>APDSVDYREKGYVTPVKNQGQCGSCWAFSSVGALEGQLKKKTGKLLNLSPQNLVDCVSENDGCGGGYMTNAFQYVQKNRGIDSEDAYPYVGQEESCMYNPTGKAAKCRGYREIPEGNEKALKRAVARVGPVSVAIDASLTSFQFYSKGVYYDESCNSDNLNHAVLAVGYGESKGNKHWIIKNSWGENWGMGGYIKMARNKNNACGIANLA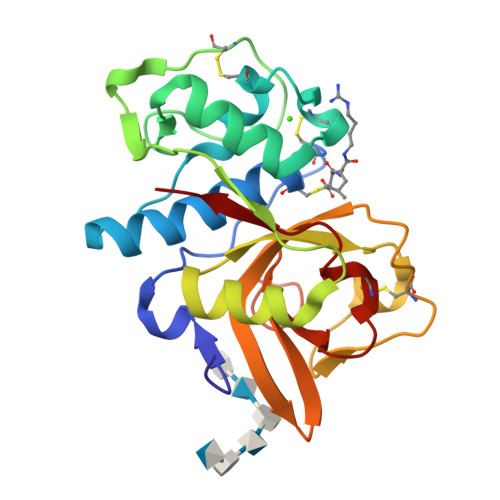SFPKM[2x]> TTCCPSIVARS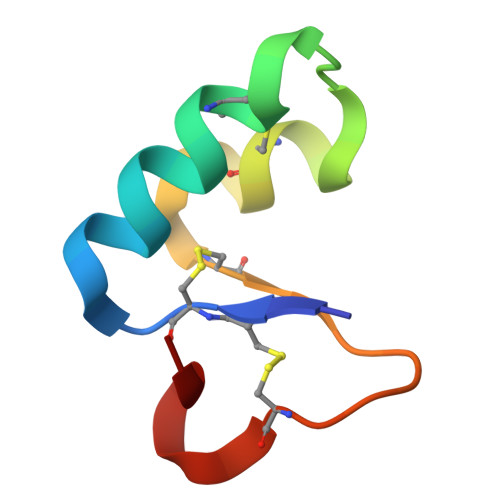NFNACRLPGTPEALCATYTGCIIIPGATCPGDYAN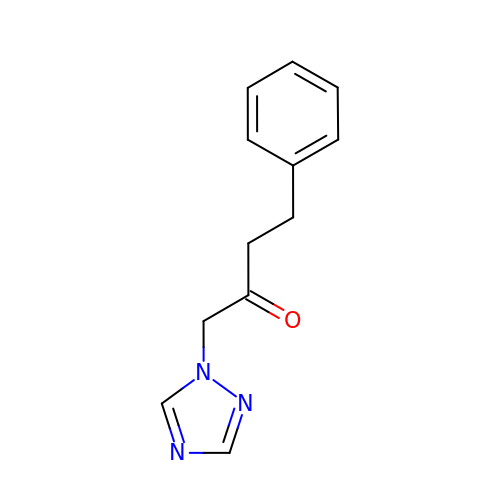4-phenyl-1-(1H-1,2,4-triazol-1-yl)butan-2-one | C12 H13 N3 O | WVMHBWUDAPTOQF-UHFFFAOYSA-N> XP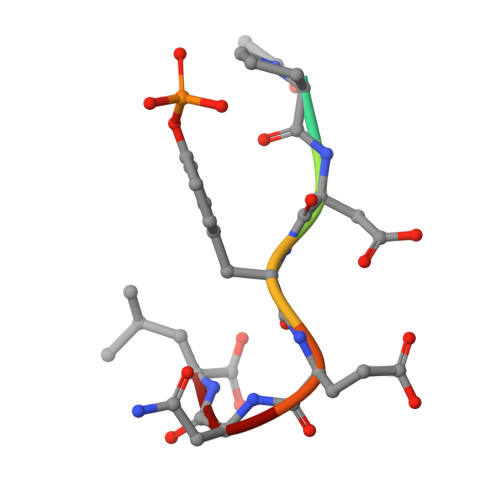DYENL> MVAKGRIIRVTGPLVVADGMKGAKMYEVVRVGELGLIGEIIRLEGDKAVIQVYEETAGVRPGEPVVGTGASLSVELGPRLLTSIYDGIQRPLEVIREKTGDFIARGVTAPALPRDKKWHFIPKAKVGDKVVGGDIIGEVPETSIIVHKIMVPPGIEGEIVEIAEEGDYTIEEVIAKVKTPSGEIKELKMYQRWPVRVKRPYKEKLPPEVPLITGQRVIDTFFPQAKGGTAAIPGPFGSGKTVTQHQLAKWSDAQVVIYIGCGERGNEMTDVLEEFPKLKDPKTGKPLMERTVLIANTSNMPVAAREASIYTGITIAEYFRDMGYDVALMADSTSRWAEALREISGRLEEMPGEEGYPAYLASKLAEFYERAGRVVTLGSDYRVGSVSVIGAVSPPGGDFSEPVVQNTLRVVKVFWALDADLARRRHFPAINWLTSYSLYVDAVKDWWHKNIDPEWKAMRDKAMALLQKESELQEIVRIVGPDALPERERAILLVARMLREDYLQQDAFDEVDTYCPPEKQVTMMRVLLNFYDKTMEAINRGVPLEEIAKLPVREEIGRMKFERDVSKIRSLIDKTN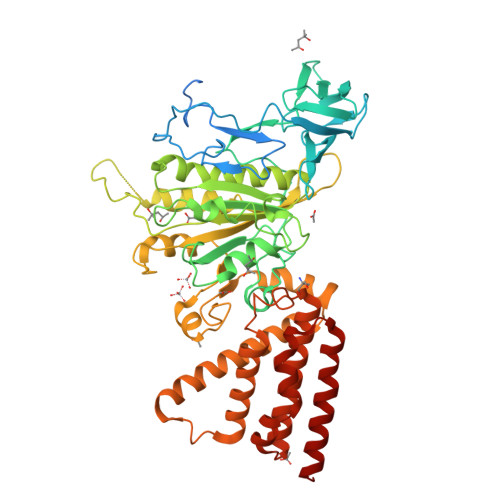EQFEELFKKYGA>ENLYFQGHMTLEIRPAVPADAEQILAFIIELADYERARHEVVTDVEGIRRSLFAEGSPTRALMCLSEGRPIGYAVFFYSYSTWLGRNGIYLEDLYVTPEYRGVGAGRRLLRELAREAVANDCGRLEWSVLDWNQPAIDFYRSIGA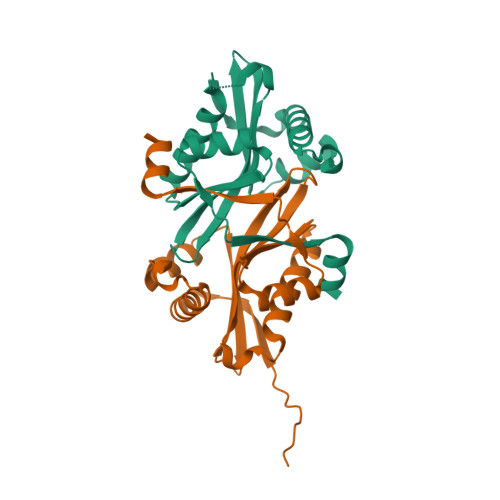LPQDEWVRYRLDGEALRKMAE[2x]>[2x]MPPQLHNGLDFSAKVIQGSLDSLPQEVRKFVEGNAQLCQPEYIHICDGSEEEYGRLLAHMQEEGVIRKLKKYDNCWLALTDPRDVARIESKTVIITQEQRDTVPIPKSGQSQLGRWMSEEDFEKAFNARFPGCMKGRTMYVIPFSMGPLGSPLAKIGIELTDSPYVVASMRIMTRMGTSVLEALGDGEFIKCLHSVGCPLPLKKPLVNNWACNPELTLIAHLPDRREIISFGSGYGGNSLLGKKCFALRIASRLAKEEGWLAEHMLILGITNPEGKKKYLAAAFPSACGKTN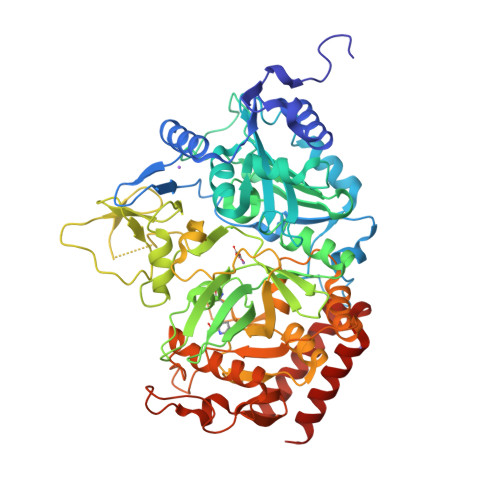LAMMNPTLPGWKVECVGDDIAWMKFDAQGNLRAINPENGFFGVAPGTSVKTNPNAIKTIQKNTIFTNVAETSDGGVYWEGIDEPLAPGVTITSWKNKEWRPQDEEPCAHPNSRFCTPASQCPIIDPAWESPEGVPIEGIIFGGRRPAGVPLVYEALSWQHGVFVGAAMRSEATAAAEHKGKVIMHDPFAMRPFFGYNFGKYLAHWLSMAHRPAAKLPKIFHVNWFRKDKNGKFLWPGFGENSRVLEWMFGRIEGEDSAKLTPIGYVPKEDALNLKGLGDVNVEELFGISKEFWEKEVEEIDKYLEDQVNADLPYEIERELRALKQRISQM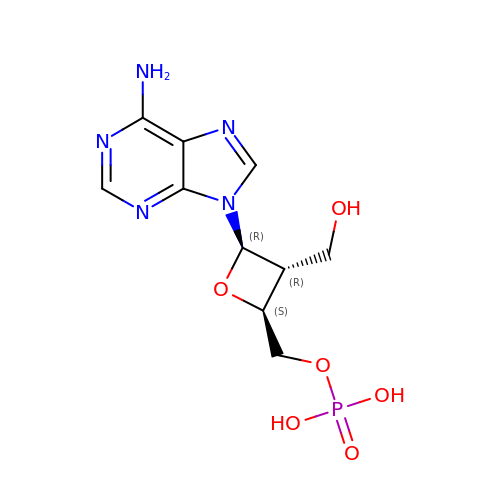[(2S,3R,4R)-4-(6-amino-9H-purin-9-yl)-3-(hydroxymethyl)oxetan-2-yl]methyl dihydrogen phosphate | C10 H14 N5 O6 P | YHDKOVKCJODYNM-OXOINMOOSA-N Using Arabidopsis thaliana Pdx1, an enzyme involved in vitamin B6 biosynthesis, and lysozyme, we demonstrate crystal scaling to suitable dimensions and numbers for time-resolved serial crystallography. Here, we report the use of droplet miniaturization for the controlled production of uniform crystals, providing an avenue for controlled substrate addition and synchronous reaction initiation. The approach was evaluated using two enzymatic systems, yielding 3 µm crystals of lysozyme and 2 µm crystals of Pdx1, an Arabidopsis enzyme involved in vitamin B6 biosynthesis. The method was demonstrated with lysozyme and Pdx1, with crystals grown in droplets producing equivalent (if not better) diffraction data quality to those produced under batch conditions.

We show that with diminishing volumes, nucleation becomes improbable, but this can be countered by seeding. A seeding strategy was used to overcome the improbability of Pdx1 nucleation occurring with diminishing droplet volumes. Pdx1 and trypsin I droplet preparations required the use of seeds within the mother liquor. In droplets a 2:1 mixture of seeds (107 ml−1) diluted in mother liquor with 12 mg ml−1 Pdx1 was used. At low picolitre and femtolitre scales, nucleation becomes improbable and can be bypassed using a seeding strategy for producing crystals only a few micrometres in length. Droplets were collected in microcentrifuge tubes and stored at room temperature for 2–3 days with a mineral oil overlay to prevent coalescence. Crystals were retrieved from droplets by a procedure called ‘breaking the emulsion’. Lysozyme and Pdx1 crystals were concentrated by settling and applied to sheet-on-sheet (SOS) chips. Serial synchrotron crystallography (SSX) data for lysozyme and Pdx1 crystals grown in batch and within microfluidic droplets were collected on the new ID29 beamline at the European Synchrotron Radiation Facility (ESRF, France) using a 2 × 4 µm (V × H) beam of 11.56 keV X-rays, with a 90 µs pulse and 231.25 Hz repetition rate, and a 20 µm step movement between images. A JUNGFRAU 4M detector with a sample-to-detector distance of 175 mm (1.8 Å in the corner) was used to collect diffraction patterns.

>[4x]MEGTGVVAVYGNGAITEAKKSPFSVKVGLAQMLRGGVIMDVVNAEQARIAEEAGACAVMALERVPADIRAQGGVARMSDPQMIKEIKQAVTIPVMAKARIGHFVEAQILEAIGIDYIDESEVLTLADEDHHINKHNFRIPFVCGCRNLGEALRRIREGAAMIRTKGEAGTGNIIEAVRHVRSVNGDIRVLRNMDDDEVFTFAKKLAAPYDLVMQTKQLGRLPVVQFAAGGVATPADAALMMQLGCDGVFVGSGIFKSGDPARRARAIVQAVTHYSDPEMLVEVSCGLGEAM> GAQPNLGRSTKATPDFPTHFPKSSIGIENELAGLVVAMPANSAQKFGYVKSAQGDALFMLTKDMNQGSYQRPPSLQDGKNYQNWQTHTVELVSYPCEMDDKAAVETRKQAMLWLATHFTTHIDQSNHQPLAPIQSEDGRFVIEITNAKHVIAAGNGISAESQGQTITMTPSGQQATVGVAAKGFGTSATPELRLLESAPWYQKSLKSQFASLTSAENLDDKELAANVFAYLTSIYLKTAELAKKFGIYINEWDPMSEQITPNANGLTDPKVKNAWEILPRTKPSKIVEILSKSDAKAVMKHIKPQLQSRYSESLSKNVFQYFQDGGEVAGHG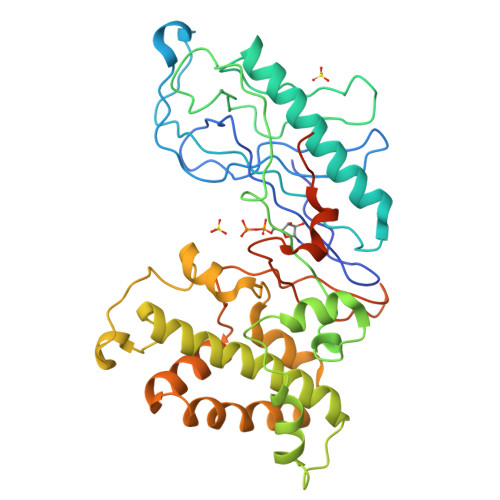INNATVGDKHSPELAILFEFRTVPNELQSYLPKTESTTKSEVKLLDQFDPMKRKTVIQQVESLV> GSMAPLGGAPRLVLLFSGKRKSGKDFVTEALQSRLGADVCAVLRLSGPLKEQYAQEHGLNFQRLLDTSTYKEAFRKDMIRWGEEKRQADPGFFCRKIVEGISQPIWLVSDTRRVSDIQWFREAYGAVTQTVRVVALEQSRQQRGWVFTPGVDD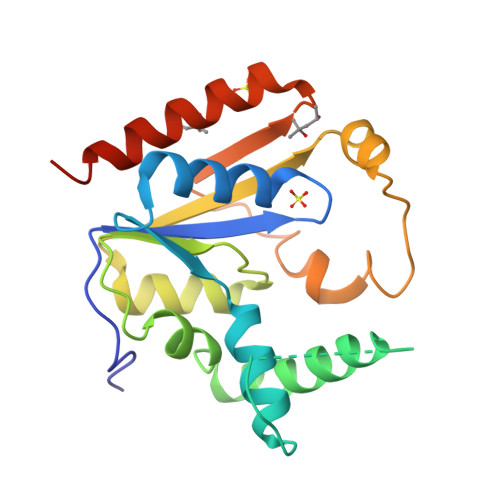AESECGLDNFGDFDWVIENHGVEQRLEEQLENLIEFIRSRLKLHHHHHH>[2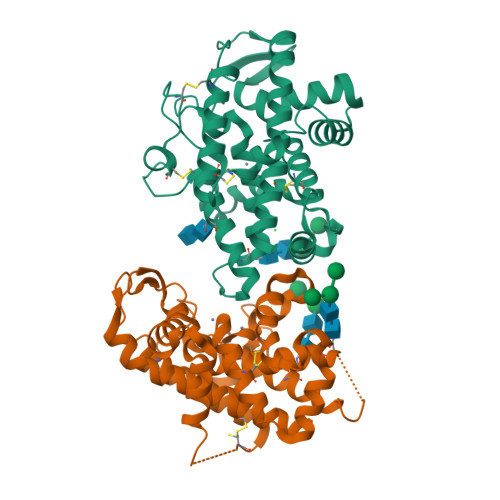x]WSKEGHVMTCRIAQGLLNDEAAHAVKMLLPEYVNGDLSALCVWPDQVRHWYKYKWTSPLHFIDTPDKACNFDYERDCHDQHGVKDMCVAGAIQNFTTQLSHYREGTSDRRYNMTEALLFLSHFMGDIHQPMHVGFTSDAGGNSIDLRWFRHKSNLHHVWDREIILTAAKDYYAKDINLLEEDIEGDFTDGIWSDDLASWRECGNVFSCVNKFATESINIACKWGYKGVEAGETLSDDYFNSRLPIVMKRVAQGGIRLAMLLNNVFGASQQEDSVVAT> MAWVTQAYSSGLSQNSIISLTGNDRTVADGTFNSMIMPRAVIANEREHFMKTRIDKIEHDLNRSAKQEMMDRQSLAEDYNALNLAVGQEIKLDIATQHQLNRLGSAMYKADHERETELTDLINRIRENEVTVNGILENQKAITAAERADLLLEVVASTAKSVSAAGRAAADGSGVVPVFGPSVANGIKVGIDIADSVAEAAIAVKESGIITQLNDVYHAFQSVHVAPNDVIKPAAVVAGTSTELIGNLQAIYSRLRSHSDIGFKKATVGDVIPNSYMIKPVNSTEYASWQLYVIHPVQGSLGLVVQLMGDALTYNVFAQYGNTSASEFGKTVLTGGATNTALEGTKVKFQTKVTAQQALALTMALKDAASMLSQGELIGYFEQYINLALEPDNLSLQDNMHKYHHLLTSQNSPIDWNYHDEEMHKWLDSRKTTNYDAMQKKDGTVIADIHIPKVFNDLRNTTLHCKLEGKQTIAGYTVYEYLIGPWAHYGDIDYSVVVDTLNEETKWYCEVIGIDGHLLIEKSVQHKPEKILELTVNDSGVTSFNGRNHDRLKLKVYVKDSLSVKVFRNWIGINAPRVKTK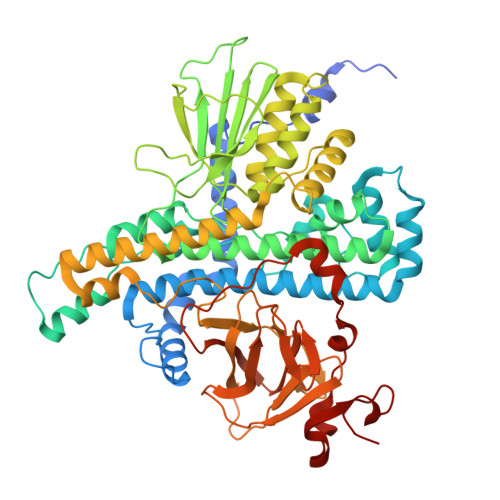MFNDHIGVKYDYSHFDKNISPAHLTLTDLGWHTWDQYNAGNWTNIKP> GSHMYIGPEVPKEDLIWQDPLPQPIYNPTEQDIIDLKFAIADSGLSVSELVSVAWASASTFRGGDKRGGANGARLALMPQRDWDVNAAAVRALPVLEKIQKESGKASLADIIVLAGVVGVEKAASAAGLSIHVPFAPGRVDARQDQTDIEMFELLEPIADGFRNYRARLDVSTTESLLIDKAQQLTLTAPEMTA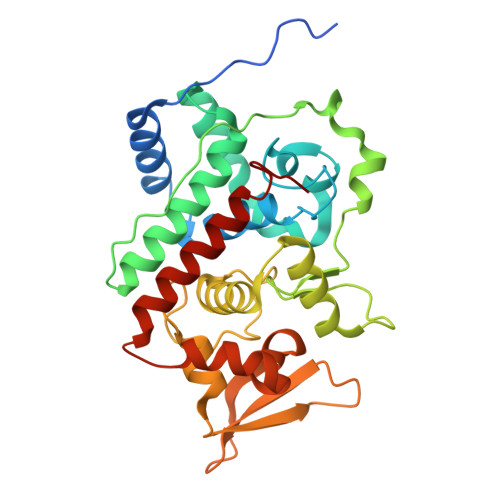LVGGMRVLGANFDGSKNGVFTDRVGVLSNDFFVNLLDMRYEWKATDESKELFEGRDRETGEVKFTASRADLVFGSNSVLRAVAEVYASSDAHEKFVKDFVAAWVKVMNLDRFDLL>[4x]AGITGTWYNQLGSTFIVTAGADGALTGTYESAVGNAESRYVLTG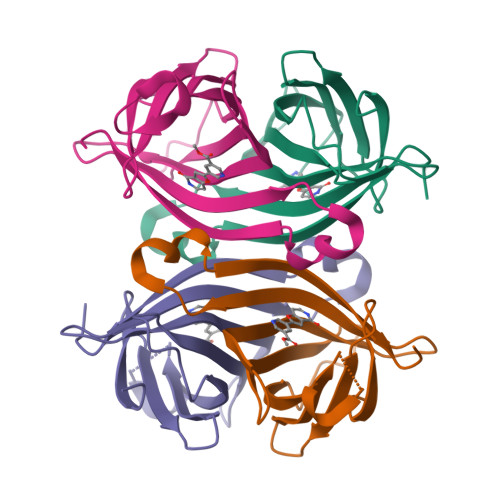RYDSAPATDGSGTALGWTVAWKNNYRNAHSATTWSGQYVGGAEARINTQWLLTSGTTEANAWKSTLVGHDTFTKVKP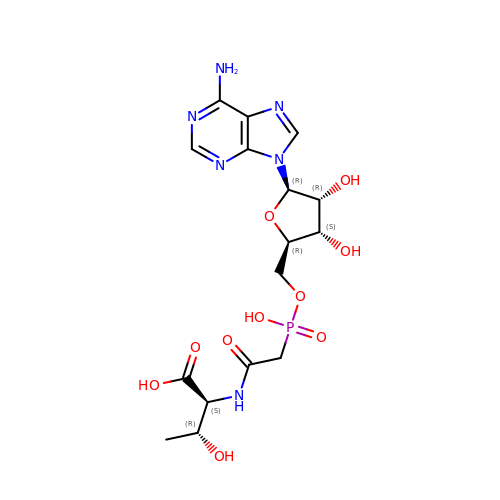(2~{S},3~{R})-2-[2-[[(2~{R},3~{S},4~{R},5~{R})-5-(6-aminopurin-9-yl)-3,4-bis(oxidanyl)oxolan-2-yl]methoxy-oxidanyl-phosphoryl]ethanoylamino]-3-oxidanyl-butanoic acid | C16 H23 N6 O10 P | DWVLLSYZUNNOOL-JOHRSRDASA-N>DPFTMMILKIGGSVITDKSAYRTARTYAIRSIVKVLSGIEDLVCVVHGGGSFGHIKAMEFGLPGPKNPRSSIGYSIVHRDMENLDLMVIDAMIEMGMRPISVPISALRYDGRFDYTPLIRYIDAGFVPVSYGDVYIKDEHSYGIYSGDD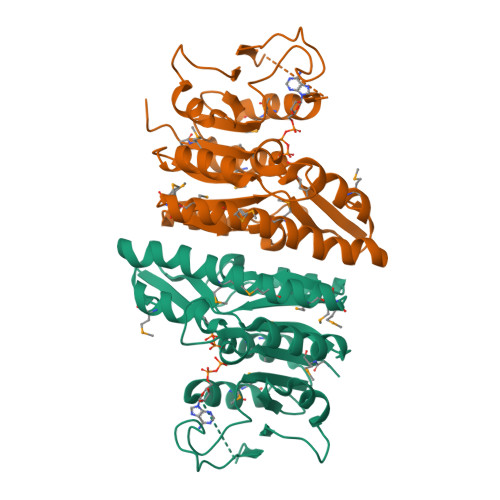IMADMAELLKPDVAVFLTDVDGIYSKDPKRNPDAVLLRDIDTNITFDRVQNDVTGGIGKKFESMVKMKSSVKNGVYLINGNHPERIGDIGKESFIGTVIR[4x]>MGTATDNARQVTIIGAGLAGTLVARLLARNGWQVNLFERRPDPRIETGARGRSINLALAERGAHALRLAGLEREVLAEAVMMRGRMVHVPGTPPNLQPYGRDDSEVIWSINRDRLNRILLDGAEAAGASIHFNLGLDSVDFARQRLTLSNVSGERLEKRFHLLIGADGCNSAVRQAMASVVDLGEHLETQPHGYKELQITPEASAQFNLEPNALHIWPHGDYMCIALPNLDRSFTVTLFLHHQSPAAQPASPCFAQLVDGHAARRFFQRQFPDLSPMLDSLEQDFEHHP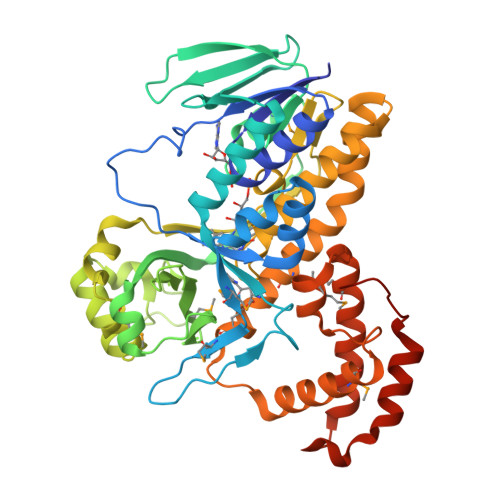TGKLATLRLTTWHVGGQAVLLGDAAHPMVPFHGQGMNCALEDAVALAEHLQSAADNASALAAFTAQRQPDALAIQAMALENYVEMSSKVASPTYLLERELGQIMAQRQPTRFIPRYSMVTFSRLPYAQAMARGQIQEQLLKFAVANHSDLTSINLDAVEHEVTRCLPPLSHLCAAALEHHHHHH[2x]>MPTLFDPIDFGPIHAKNRIVMSPLTRGRADKEAVPAPIMAEYYAQRASAGLIITEATGISREGLGWPFAPGIWSDAQVEAWKPIVAGVHAKGGKIVCQLWHMGRMVHSSVTGTQPVSSSATTAPGEVHTYEGKKPFEQARAIDAADISRILNDYENAARNAIRAGFDGVQIHAANGYLIDEFLRN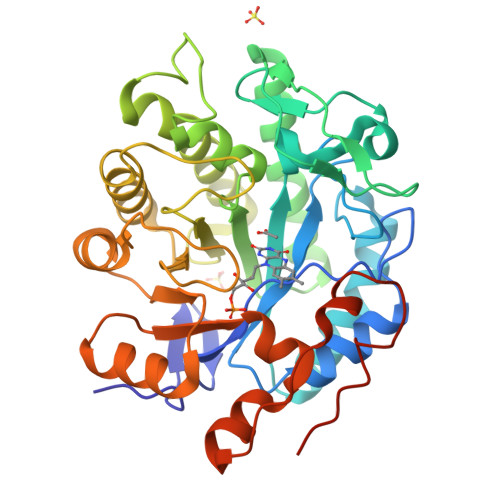GTNHRTDEYGGVPENRIRFLKEVTERVIAAIGADRTGVRLSPNGDTQGCIDSAPETVFVPAAKLLQDLGVAWLELREPGPNGTFGKTDQPKLSPQIRKVFLRPLVLNQDYTFEAAQTALAEGKADAIAFGRKFISNPDLPERFARGIALQPDDMKTWYSQGPEGYTDYPSATSGPNLEHHHHHH[4x]> MGAPEEMPVDRILEAELAVEQKSDQGVEGPGGTGGSGSSPNDPVTNICQAADKQLFTLVEWAKRIPHFSSLPLDDQVILLRAGWNELLIASFSHRSI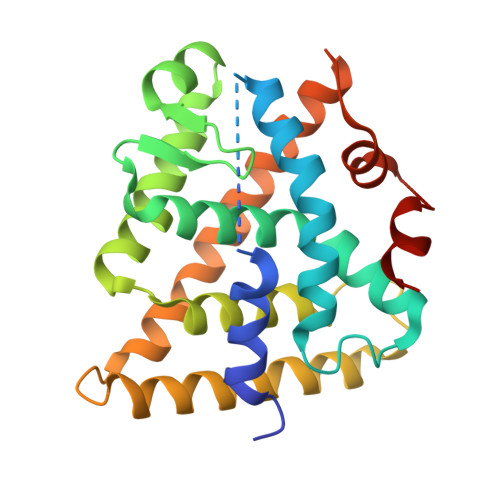DVRDGILLATGLHVHRNSAHSAGVGAIFDRVLTELVSKMRDMRMDKTELGCLRAIILFNPDAKGLSNPSEVEVLREKVYASLETYCKQKYPEQQGRFAKLLLRLPALRSIGLKCLEHLFFFKLIGDTPIDTFLMEMLEAGSGSGSHKILHRLLQDSSS> IV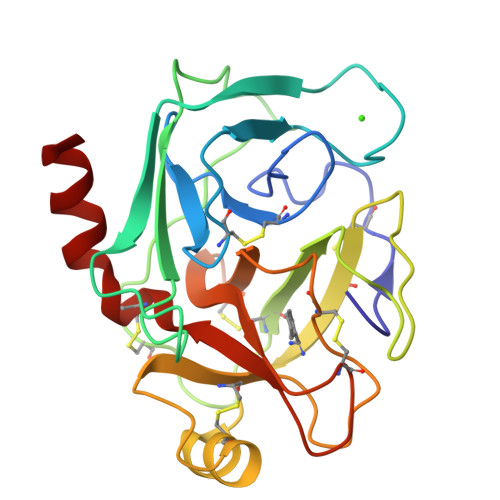GGYTCQENSVPYQVSLNSGYHFCGGSLINDQWVVSAAHCYKSRIQVRLGEHNINVLEGNEQFVNAAKIIKHPNFDRKTLNNNIMLIKLSSPVKLNARVATVALPSSCAPAGTQCLISGWGNTLSSGVNEPDLLQCLDAPLLPQADCEASYPGKITDNMVCVGFLEGGKDSCQGDSGGPVVCNGELQGIVSWGYGCALPDNPGVYTKVCNYVDWIQDTIAAN>MDIGINSDPHHHHHHGGLDIVNNATGDDNRDDLNIRTYGATETSSLIMLRARGTASAPAAVQTGDRLGGVLFRGWNGTAWMGSGQILSVAEENFTTAVKTNLQFHVGG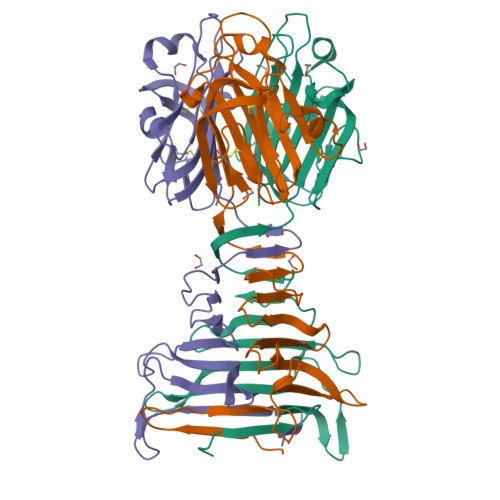AGEAMRISNTGNVGIGTTTTTEKLNVQGNVAVSGEITSVRSWGIKRGPTSFSANYINVWNSGYHVGSSIDCTTSTTGCRILKAGTYEIRCVQRAGTSGNSVYVGIALNGDRTALESRNDVLWNHSHTAYSGSYTESNFMGTLSANDLITCGAPVNTMAADLVYAVPAYNGTMQIKRVD[3x]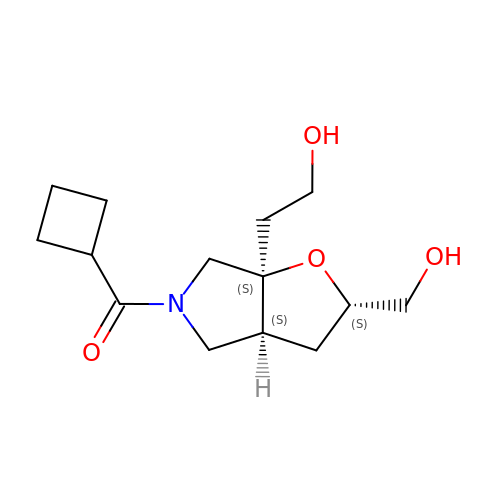cyclobutyl[(2S,3aS,6aS)-6a-(2-hydroxyethyl)-2-(hydroxymethyl)hexahydro-5H-furo[2,3-c]pyrrol-5-yl]methanone | C14 H23 N O4 | LOAFEZNLOIOHIT-SGMGOOAPSA-N RNA guanine-7 methyltransferase (RNMT) catalyses the transfer of a methyl group from S-adenosylmethionine (SAM) to the cap intermediate to form the cap m7G(5′)ppp(X) and the by-product S-adenosylhomocysteine (SAH). RNMT was identified based on homology to the yeast and viral homologues and in vitro activity. This basic cap structure (cap 0, m7G(5′)ppp(X)) protects RNA from degradation by nucleases during synthesis and recruits factors involved in RNA processing and translation initiation. RNMT has an activating co-factor RNMT-activating miniprotein (RAM) clamped at the interface of the catalytic domain and the modular lobe 416–456. Consequently, RNMT is a target of interest in cancers and immune disorders.

Since attempts to crystallise RNMT with the G(5′)ppp(5′)G (cap) had been unsuccessful, we co-crystallised RNMT with the cap surrogate, GMP-PnP. GMP-PnP was confirmed as a cap competitive inhibitor with a Ki of 2.3 µM (0.9–5.5 µM). Crystallisation of RNMT with GMP-PnP provides the first structural characterisation of a Class I methyltransferase in a complex with a cap analogue and Sinefungin. HsRNMT–Sinefungin–GMP-PnP, HsRNMT–SAH–DDD1060606 and HsRNMT–SAH–DDD1870799 co-complexes were solved, respectively, at 2.5, 2.0 and 2.4 Å in space group P21. The Sinefungin molecule is well resolved in the electron density map for both chains of the asymmetric unit and shares a common network of interaction to that observed for SAH binding to HsRNMT. GMP-PnP was successfully built in just one of the chains in the asymmetric unit and is located between the α-helix A and the β-strands 8/9. When co-crystallised with HsRNMT and Sinefungin, the GMP-PnP guanine moiety is stabilised within the cap pocket by hydrogen bonds to residues H288, Y289, E370, Y467 and the Sinefungin 5-amino group, as well as through a Pi-stacking interaction with F285. The GMP-PnP ribose makes two hydrogen bonds with N176, whereas the beta-gamma pyrophosphate group interacts with the polypeptide chain via two salt bridges to K208. Finally, the distance measured between the Sinefungin 5-amino group and the guanine N7 (2.4 Å) alongside the angle formed by C5/5-NH2/N7 (140°) confirms that GMP-PnP is observed in an ideal orientation to permit the methyl transfer, similar to the predicted model published. SAH and Sinefungin are stabilised in the active site through an identical network of hydrogen bonds, involving residues K180, G205, D227, D261, S262 and Q284, as well as 2 salt bridges with K180. These results support the hypothesis that Sinefungin binds in the SAM-binding site in the presence or absence of the cap.

>[2x]SQSRIFYLRNFNNWMKSVLIGEFLEKVRQKKKRDITVLDLGCGKGGDLLKWKKGRINKLVCTDIADVSVKQCQQRYEDMKNRRDSEYIFSAEFITADSSKELLIDKFRDPQMCFDICSCQFVCHYSFESYEQADMMLRNACERLSPGGYFIGTTPNSFELIRRLEASETESFGNEIYTVKFQKKGDYPLFGCKYDFNLEGVVDVPEFLVYFPLLNEMAKKYNMKLVYKKTFLEFYEEKIKNNENKMLLKRMGLGCLSKSEWEATSIYLVFAFEKQQ>[2x]VPHKSSLPEGIRPGTVLRIRGLVPPNASRFHVNLLCGEEQGSDAALHFNPRLD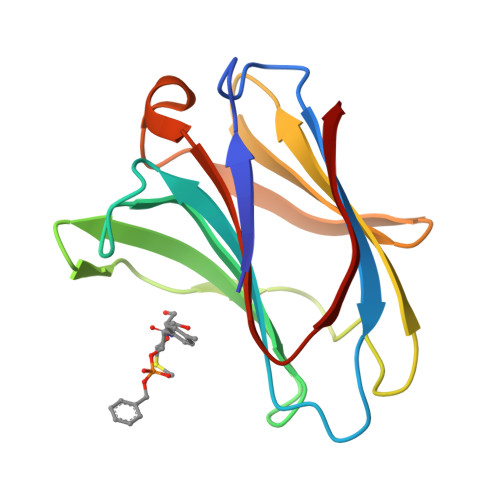TSEVVFNSKEQGSWGREERGPGVPFQRGQPFEVLIIASDDGFKAVVGDAQYHHFRHRLPLARVRLVEVGGDVQLDSVRIF> MAEVLKKSGVIYGDDVRKLFDYAQEKGFAIPAINVTSSSTVVAALESARDNKSPIILQTSQGGAAYFAGKGVSNSDQTASIQGSIAAAHYIRAISPVYGIPVILHTDHCAKKLLPWFDGMLKADEEFFAKTGQPLFSSHMLDLSEETDDENIATCVKYFERMSKMNQWLEMEIGITGGEEDGVNN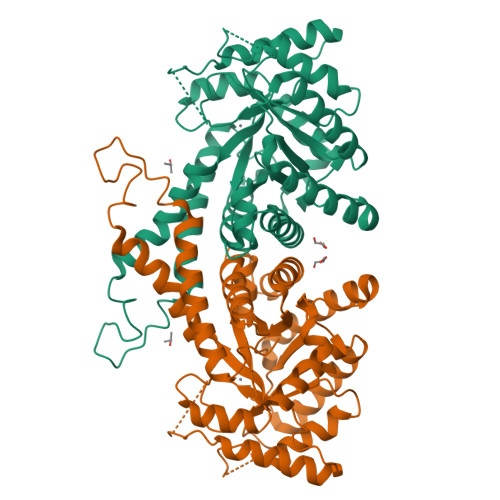EHVEKESLYTQPETVFAVYKALAPISPNFSIAAAFGNVHGVYKPGNVQLRPSILGEHQKYAKEQIGTDNKKPLYLVFHGGSGSSQEEFDTAIASGVVKVNLDTDCQYAYLTGIRDYILNKKEYLMTPVGNPDGEDKPNKKYFDPRVWVREGEKSMSARIAEALEIFHTKNQL> MDKVLNREESLQL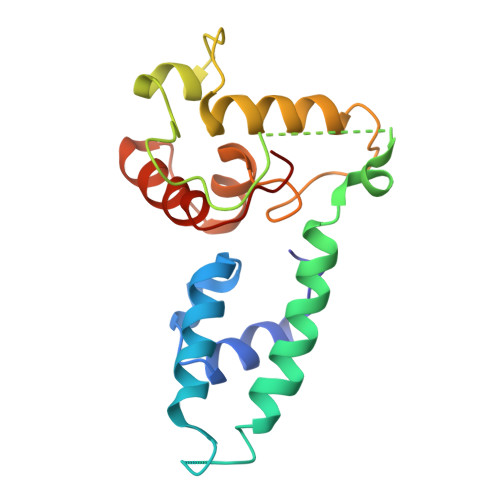MDLLGLERSAWGNIPLMRKAYLKKCKEFHPDKGGDEEKMKKMNTLYKKMEDGVKYAHQPDFGGFWDATEVFASSLNPGVDAIYCKQWPECVKKMSTNCICLLCLLRMKHENRKLYRKDPLVWVDCYCFDCFRMWFGLDLCEGTLLLWCDIIGQTTYRDLKL> MDSLDQCIVNACKNSWDKSYLAGTPNKDNCSGF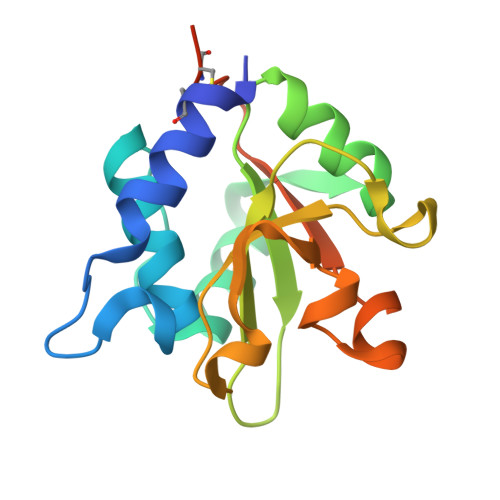VQSVAAELGVPMPRGNANAMVDGLEQSWTKLASGAEAAQKAAQGFLVIAGLKGRTYGHVAVVISGPLYRQKYPMCWCGSIAGAVGQSQGLKSVGQVWNRTDRDRLNYYVYSLASCSLPRASLEHHHHHH>MTDFYTIKDAQADLAIAPLNLTVLLAPYSTTPATTLESPTDGSLAIPPGYKSVGHFEKQAGL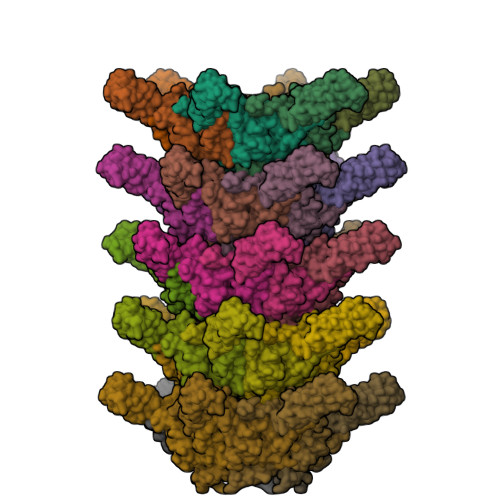TLGNEFDSKDIEAYGEPEPIRTIINKRTTTFDFAMYQNQRNVLELIWTQDFSNIQPSEFGGIVLEAPKVPKNIYYRAILVGMDDRNDRPIWLYWLMPKVKLDKLDNQTLNDDNVIEYKPTLKAFRDDVVGYSVAQGFAGPGWRDLVATAGFGEALTALTITPGSPTVTVATGASHTAQLLVEGDNGINYTPDVVFTSSAPDKASVSAAGLVTGVAAGSATITATKGALTATATVTVTA[30x]MBH reactions are valuable carbon-carbon bond forming transformations in organic synthesis, for which no natural enzymes are known. Previous work has afforded the MBHase BH32.1413 which promotes catalysis via a histidine nucleophile. In this work, His23 is replaced by Nδ-methylhistidine (MeHis) for the creation of a more efficient MBHase. In this study, we explore the evolutionary trajectory of a BH32 variant with MeHis in place of His23.

Following evaluation of >18,000 clones, a BHMeHis1.8 variant emerged containing 23 mutations. More detailed kinetic characterization of BHMeHis1.8 reveals a kcat of 4.5 ± 0.19 min−1, making it 13-fold more active than our previously engineered MBHase BH32.14 (0.35 ± 0.03 min−1) and 2000-fold more active than the original BH32 design (0.13 ± 0.01 h−1). During evolution of BHMeHis1.8, Arg124, which was essential to catalysis in BH32.1413, was replaced by a tryptophan. To gain insights into this mechanism, crystal structures of apo-BHMeHis1.0 and apo-BHMeHis1.8 were solved. Efforts to obtain structures complexed with either substrate(s) or product have thus far been unsuccessful. Comparison of the BHMeHis1.8 and BHMeHis1.0 structures reveals that the 23 mutations installed during evolution cause minimal changes to the overall protein fold (secondary structure root mean square deviation (rmsd) 0.47 Å, Supplementary Fig. 9). The MeHis nucleophile adopts a single conformation in the structures of BHMeHis1.8 and BHMeHis1.0, however a notable 120° rotation of the imidazole ring has occurred. In BHMeHis1.8, MeHis23 is positioned by an adjacent Trp42 residue installed during evolution. Molecular docking of (R)-3 into the apo-BHMeHis1.8 structure reveals a binding mode with the aromatic nitrobenzene ring sandwiched between Trp124 and Phe132 and the polar 1,3-hydroxyketone motif pointing towards a newly introduced Glu26. Interestingly, a PROPKA 331 calculation based on apo-BHMeHis1.8 predicts that Glu26 has an unusually high pKa of 8.1, likely due to its positioning within a hydrophobic environment surrounded by non-polar sidechains. Instead, Glu26 has emerged, which mediates a rate-limiting proton transfer step to deliver an enzyme (BHMeHis1.8) that is more than an order of magnitude more active than our earlier MBHase.

> MIRAVFFDSLGTLISVEGAYKIHVKEMEEVLGDYPLNPRTLWDEFDKLFKEAFSNYAGKPYRPARFILEEVMRKLAEKYGFKYPGNLQEIGVRMARRYGGLYPEVVEVLKSLKGKYHVGVILNWDTENATAFLDALGIKDLFDSITTSEEAGFAYPHPRILELALKKAGVKGEKAVYVGDNPVKDAGGSKNLGMTSILLDRKGEKREFWDKADFRVSDLREVIKIVDELNGQGSLEHHHHHH> DDKMDYDFKVKLSSERERVEDLFEYEGCKVGRGTYGHVYKAKRKDGKDDKDYALKQIEGTGISMSACREIALLRELKHPNVISLQKVFLSHADRKVWLLFDYAEHDLWHIIKFHRASKANKKPVQLPRGMVKSLLYQILDGIHYLHANWVLHRDLKPANILVMGEGPERGRVKIADMGFARLFNSPLK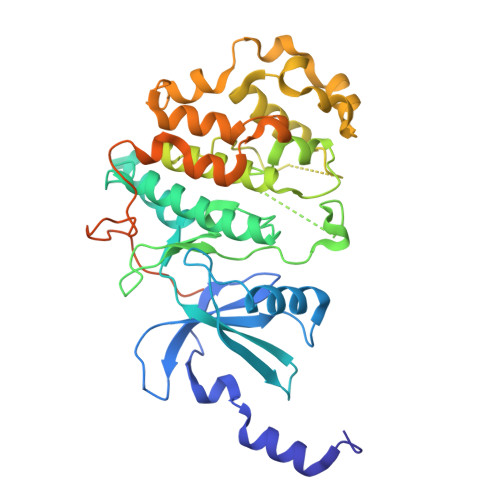PLADLDPVVVTFWYRAPELLLGARHYTKAIDIWAIGCIFAELLTSEPIFHCRQEDIKTSNPYHHDQLDRIFNVMGFPADKDWEDIKKMPEHSTLMKDFRRNTYTNCSLIKYMEKHKVKPDSKAFHLLQKLLTMDPIKRITSEQAMQDPYFLEDPLPTSDVFAGCQIPYPKREFLTEEEPDDKGDKKNQQQQQGNNHTNGTGHPGNQDSSHTQGPPLKKV>[2x]MNLPTAQEVQGLMARYIELVD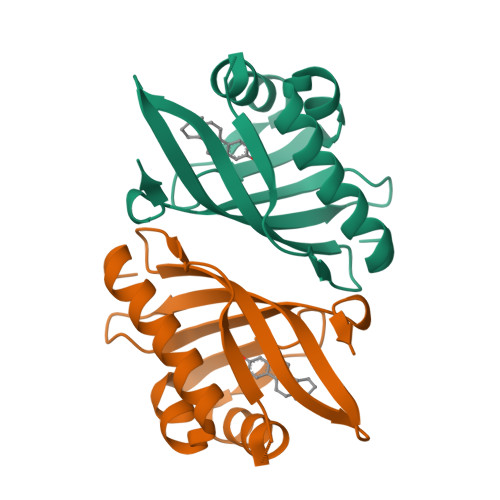VGDIEAIVQMYADDATVENPFGQPPIHGREQIAAFYRQGLGGGKVRACLTGPVRASHNGCGAMPFRVEMVWNGQPCALDVIEVMRFDEHGRIQTMQAYWSEVNLSVREPQ>[4x]MRDYSELEI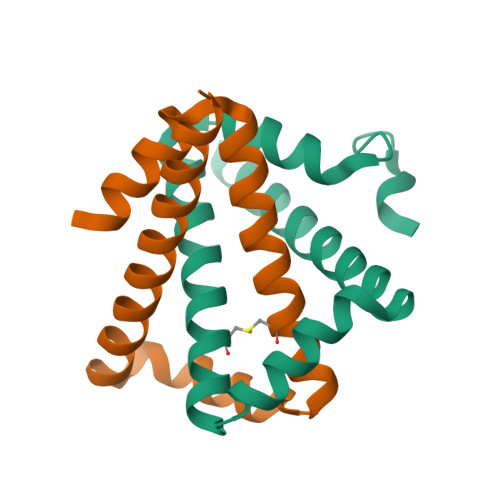FEGNPLDKWNDIIFHASKKLSKKELERLLELLALCETFIEKEDLEEKFESFAKALRIDEELQQKIESRKTDIVIQSMANILSGLEHHHHHH> MDLAKLGLKEVMPTKINLEGLVGDHAFSMEGVGEGNILEGTQEVKISVTKGAPLPFAFDIVSVAFTYGNRAYTGYPEEISDYFLQSFPEGFTYERNIRYQDGGTAIVKSDISLEDGKFIVNVDFKAKDLRRMGPVMQQDIVGMQPSYESMYTNVTSVIGECIIAFKLQTGKHFTYHMRTVYKSKKPVETMPLYHFIQHRLVKTNVDTASGYVVQHETA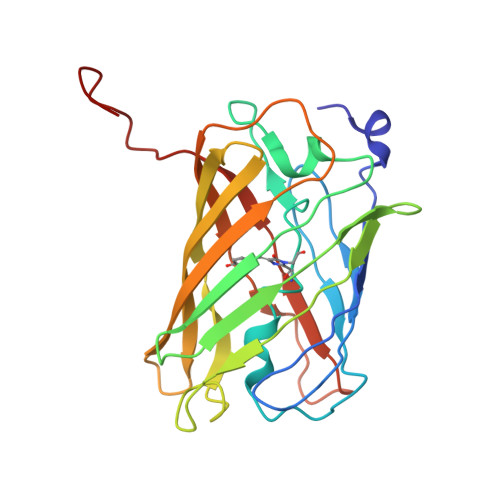IAAHSTIKKIEGSLP>MLSRKGIIPEEYVLTRLAEDPTEPRYRTRERRARFVSKKGNCNVAHKNIREQGRFLQDVFTTLVDLKWPHTLLIFTMSFLCSWLLFAMVWWLIAFAHGDLAPGEGTNVPCVTSIHSFSSAFLFSIEVQVTIGFGGRMVTEECPLAILILIVQNIVGLMINAIMLGCIFMKTAQAHRRAETLIFSKHAVITPRHGRLCFMLRVGDLRKSMIISATIHMQVVRKTTSPEGEVVPLHQVDIPMENGVGGNSIFLVAPLIIYHVIDSNSPLYDLAPSDLHHHQDLEIIVILEGVVETTGITTQARTSYLADEILWGQRFVPIVAEEDGRYSVDYSKFGNTVKVPTPLCTARQLDEDRSLLDALTLASSRGPLRKRSVAVAKAKPKFSISPDSLS[4x];>MPLAFCGTENHSAAYRVDQGVLNNGCFVDALNVVPHVFLLFITFPILFIGWGSQSSKVHIHHSTWLHFPGHNLRWILTFILLFVLVCEIAEGILSDGVTESRHLHLYMPAGMAFMAAITSVVYYHNIETSNFPKLLIALLIYWTLAFITKTIKFVKFYDHAIGFSQLRFCLTGLLVILYGMLLLVEVNVIRVRRYIFFKTPREVKPPEDLQDLGVRFLQPFVNLLSKGTYWWMNAFIKTAHKKPIDLRAIAKLPIAMRALTNYQRLCVAFDAQARKDTQSPQGARAIWRALCHAFGRRLILSSTFRILADLLGFAGPLCIFGIVDHLGKENHVFQPKTQFLGVYFVSSQEFLGNAYVLAVLLFLALLLQRTFLQASYYVAIETGINLRGAIQTKIYNKIMHMSTSNLSMGEMTAGQICNLVAIDTNQLMWFFFLCPNLWTMPVQIIVGVILLYYILGVSALIGAAVIILLAPVQYFVATKLSQAQRTTLEHSNERLKQTNEMLRGMKLLKLYAWESIFCSRVEVTRRKEMTSLRAFAVYTSISIFMNTAIPIAAVLITFVGHVSFFKESDLSPSVAFASLSLFHILVTPLFLLSSVVRSTVKALVSVQKLSEFLSSAEIREEQCAPREPAPQGQAGKYQAVPLKVVNRKRPAREEVRDLLGPLQRLAPSMDGDADNFCVQIIGGFFTWTPDGIPTLSNITIRIPRGQLTMIVGQVGCGKSSLLLATLGEMQKVSGAVFWNSNLPDSEGEDPSSPERETAAGSDIRSRGPVAYASQKPWLLNATVEENITFESPFNKQRYKMVIEACSLQPDIDILPHGDQTQIGERGINLSGGQRQRISVARALYQQTNVVFLDDPFSALDVHLSDHLMQAGILELLRDDKRTVVLVTHKLQYLPHADWIIAMKDGTIQREGTLKDFQRSECQLFEHWKTLMNRQDQELEKETVMERKASEPSQGLPRAMSSRDGLLLDEEEEEEEAAESEEDDNLSSVLHQRAKIPWRACTKYLSSAGILLLSLLVFSQLLKHMVLVAIDYWLAKWTDSALVLSPAARNCSLSQECDLDQSVYAMVFTLLCSLGIVLCLVTSVTVEWTGLKVAKRLHRSLLNRIILAPMRFFETTPLGSILNRFSSDCNTIDQHIPSTLECLSRSTLLCVSALTVISYVTPVFLVALLPLAVVCYFIQKYFRVASRD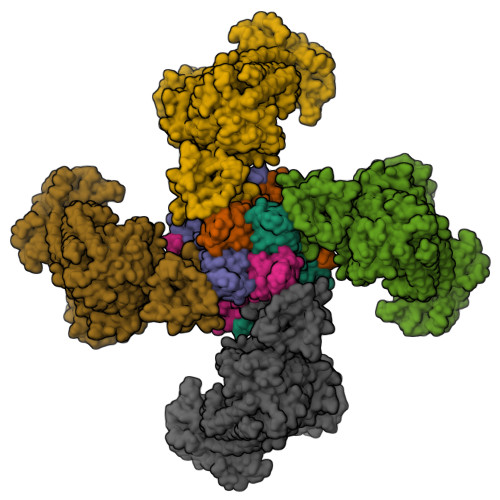LQQLDDTTQLPLVSHFAETVEGLTTIRAFRYEARFQQKLLEYTDSNNIASLFLTAANRWLEVCMEYIGACVVLIAAATSISNSLHRELSAGLVGLGLTYALMVSNYLNWMVRNLADMEIQLGAVKRIHALLKTEAESYEGLLAPSLIPKNWPDQGKIQIQNLSVRYDSSLKPVLKHVNTLISPGQKIGICGRTGSGKSSFSLAFFRMVDMFEGRIIIDGIDIAKLPLHTLRSRLSIILQDPVLFSGTIRFNLDPEKKCSDSTLWEALEIAQLKLVVKALPGGLDAIITEGGENFSQGQRQLFCLARAFVRKTSIFIMDEATASIDMATENILQKVVMTAFADRTVVTIAHRVHTILSADLVMVLKRGAILEFDKPETLLSQKDSVFASFVRADK[4x]> DKCPKGWLDFRGNCYGYFRYELPWKRAEAWCRSIRAGAHLASIHTSEEHRAIAKFISQYHHGEEEEDVWIGLFRWNSVWAWIDG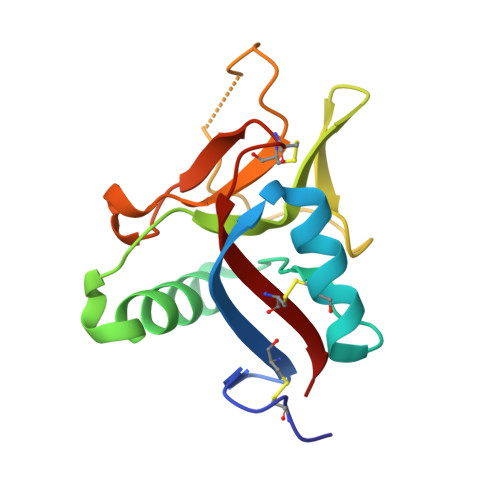SKKHYSALDDDDYPKGKHCAVLDESSGFLSWDNDSCGERNAFICKCTA>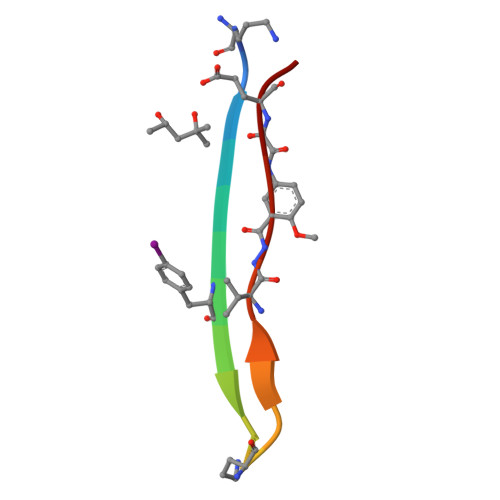[2x]AQKLVFFAEDAQKLVXED>SDKIIHLTDESFDTDVLKADGAILVDFWAEWCGPCKMIAPILDEIADEYQGKLTVAKLNIDQNPGTAPKYGIRGIPTLLLFK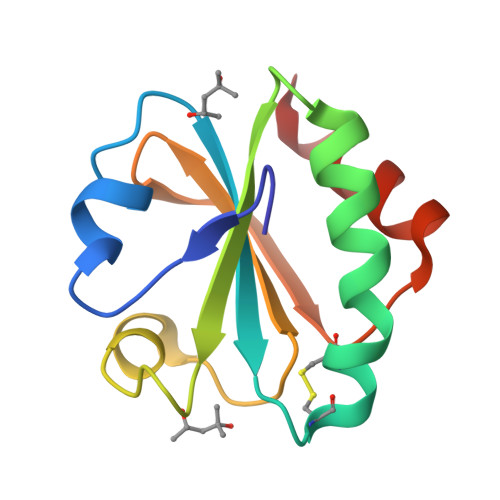NGEVAATKVGALSKGQLKEFLDANLA[2x]> SGV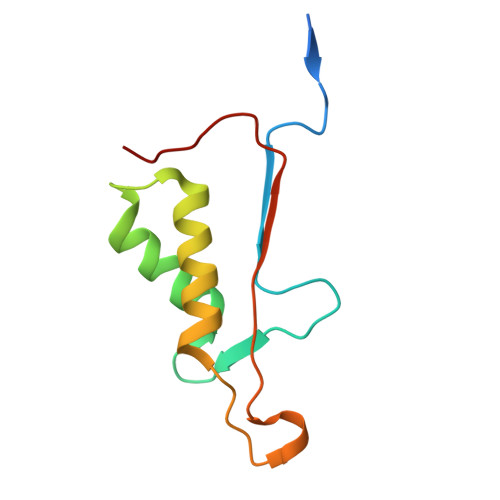DDDMACHKIPVEADFLYAYSTAPGYYSWRNSKDGSWFIQSLCAMLKQYADKLEFMHILTRVNRKVATEFESFSFDATFHAKKQIPCIVSMLTKELYFYH BMPR2 encodes for the bone morphogenetic protein (BMP) type II receptor kinase (BMPR2), which assembles with type I BMP receptor kinases to transduce BMP ligand signaling through the phosphorylation of transcription factors SMAD1/5/8. Mutations in the gene BMPR2 have emerged as the predominant risk factor accounting for some 53–86% of heritable cases and 14–35% of idiopathic cases. The type II receptor BMPR2 lacks the regulatory GS domain found in BMP type I receptors and is accepted to be constitutively active. BMPR2 shows the typical bilobal architecture of a protein kinase.

Diffracting crystals were obtained in the presence of the ligand ADP and the crystal structure was solved and refined at a resolution of 2.35 Å. Two protein molecules were present in the asymmetric unit. Both chains formed an identical interaction with Mg-ADP, but showed minor differences in the partially disordered activation loop as well as the C-terminus through which crystal contacts were formed. The structure reveals a conserved fold with other type II receptors with a pattern of specific kinase domain insertions that define the BMP/TGF-β receptor family. Consistent with this view, the kinase domain structure of BMPR2 shows an active conformation as evidenced by the correct positioning of the αC helix, as well as the catalytic residues within the ATP-binding pocket which are captured in complex with Mg-ADP. The correct positioning of the αC helix is evidenced by the 2.8 Å salt bridge formed between the catalytic residues Lys230 (β3 strand) and Glu243 (αC helix). Canonical interactions are also observed with Mg-ADP, including two hydrogen bonds with the kinase hinge region and further hydrogen bonds with the catalytic loop and phosphate-binding loop (β1-β2), also known as the glycine-rich loop. The activation loop (A-loop) makes surprisingly few contacts with the catalytic domain. However, a minor deviation from this state is apparent from some localized disorder in the activation loop. This observation potentially reflects the requirement for this flexible region to bind to the substrate type I receptor as they receptors assemble together upon extracellular ligand binding.

>MEAAASEPSLDLDNLKLLELIGRGRYGAVYKGSLDERPVAVKVFSFANRQNFINEKNIYRVPLMEHDNIARFIVGDERVTADGRMEYLLVMEYYPNGSLCKYLSLHTSDWVSSCRLAHSVTRGLAYLHTELPRGDHYKPAISHRDLNSRNVLVKNDGTCVISDFGLSMRLTGNRLVRPGEEDNAAISEVGTIRYMAPEVLEGAVNLRDCESALKQVDMYALGLIYWEIFMRCTDLFPGESVPEYQMAFQTEVGNHPTFEDMQVLVSREKQRPKFPEAWKENSLAVRSLKETIEDCWDQDAEARLTAQCAEERMAELMMIWERNKSVSPTAHHHHHH[2x]> MAVIADPETAQGFRLAGLEGYGASSAEE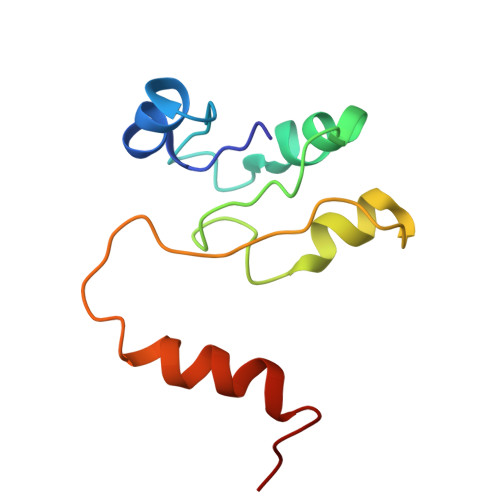AQSLLETLVERGGYALVAVDEALLPDPERAVERLMRGRDLPVLLPIAGLKEAFQGHDVEGYMRELVRKTIGF>[3x]MFKNALRRAGVAAPRISRVAQRGYAEAKATPTEVTSILEERIRGVSGEANLNETGRVLSVGDGIARVFGLNNIQAEELVEFASGVKGMALNLEAGQVGI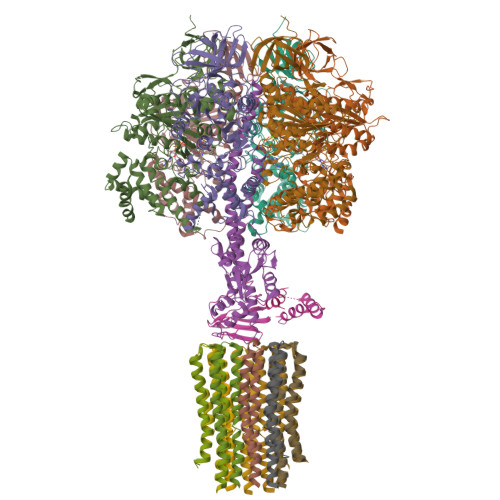VLFGSDRLVKEGETVKRSGSIVDVPVGPALLGRVVDALGNPIDGKGPIETEFRIRAQVKAPGILPRTSVNEPMQTGLKAVDALVPIGRGQRELIIGDRQTGKTQIAIDTILNQKRWNYGQDEKKKLYCVYVAVGQKRSTVAQLVQTLEHHDALKYSIIVAATASEAAPLQYLAPFTGTAMGEWFRDNGKGALIVFDDLSKQAVAYRQMSLLLRRPPGREAYPGDVFYLHSRLLERAAKMNEREGGGSLTALPIIETQGGDVSAYIPTNVISITDGQIFLEAELFYKGIRPAINVGLSVSRVGSAAQVKAMKQVAGSLKLFLAQYREVAAFAQFGSDLDASTKQTLTRGERLTLLLKQKQASPMSSEEMVPLIYAGVNGYIDNIPVKQVEKFEAEFVSYLHANESDLLKDIAATGELSKENLEKLKSITENFVGSFAK;>MVLPRLIPRLSRSAFKVAQANNRVFNAPFRGMASSAGVGSGKIRTVIGAVVDVQFEQDNLPAILNALTIDRGEGNKLVLEVAQHLGENTVRTIAMDGTEGLVRGTSVADTGAPITIPVGRGTLGRIINVCGEPIDERGPIEATKFLPIHADPPTFAEQSTTAEVLETGIKVVDLLAPYARGGKIGLFGGAGVGKTVFIQELINNIAKAHGGFSVFCGVGERTREGNDLYREMKETGVINLEGESKVTLVFGQMNEPPGARARVALTGLTIAEYFRDEEGQDVLLFVDNIFRFTQAGSEVSALLGRIPSAVGYQPTLATDMGALQERITTTQKGSVTSVQAVYVPADDLTDPAPATTFAHLDATTVLSRGISELGIYPAVDPLDSKSRLLDIDVVGQEHYDVASNVQQTLQAYKSLQDIIAILGMDELSEQDKLTVERARKIQRFLSQPFTVAEVFTGIEGRLVSLKDTVRSFKEILDGKHDALPEAAFYMVGGIEEVVAKAEKLAAESK[3x];> MFALRTAARPAARSVGATRNYATLREIEMRLKSIKNIEKITNTMKIVASTKLGKAQRAMATSKVYNEASEKVFENSETAVPENIEKRLWVVVSSDKGLCGSIHSQLARTVRRKLLDFESGEKLIDIVAVGEKIKAQLGRSNPEQMRLSFGGTGKEAPTFEEAAHIADEILALDTQYDDIEIVYNKVLSGISFEPIMKESYSAKAIEDAPKFGQYELEDDVVKNLADFSLANTIYAAMAEGHAAEISARRNAMDNASKNASDMINKYSILYNRTRQAVITNELVDIITGASSLE;> MSDHTRSQNWTNLILTQSIYNQKEVTQVNIPSTAGELGILANHVPTIQQLKPGVVEVIETNGETKSYFISGGFATVQPDSELSVNSIEAFQAEDFSPEAIKSLTAEAQKNAQSADEAVAAEAEIELEVLEALAHFAK;>[10x]MQLVLAGKYIGAGLASIGLVGAGIGIAIVFAALINGVSRNPALKGQLFTYSILGFALSEATGLFALMIAFLLLYAV>[2x]GHMKKKVWREEKERLLKMTLEERRKEYLRDYIPL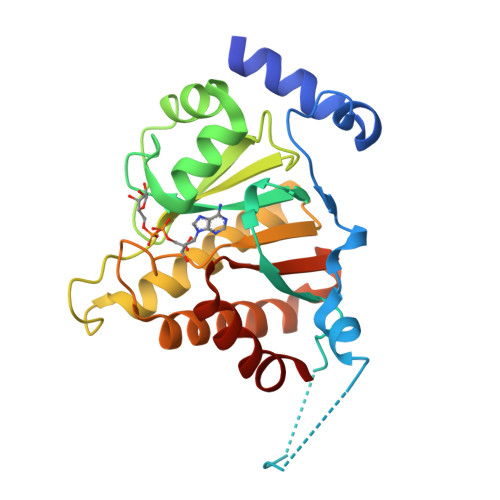NSILSWKEEMKGKGQNDEENTQETSQVKKSLTEKVSLYRGDITLLEVDAIVNAANASLLGGGGVDGCIHRAAGPCLLAECRNLNGCDTGHAKITCGYDLPAKYVIHTVGPIARGHINGSHKEDLANCYKSSLKLVKENNIRSVAFPCISTGIYGFPNEPAAVIALNTIKEWLAKNHHEVDRIIFCVFLEVDFKIYKKKMNEFFSVD The rotating flagellar filament primarily functions as a propeller, acting as an Archimedean screw, and supercoiling of the filament is essential as rotations of a straight filament do not generate thrust. Here, we show the atomic cryo-electron microscopy structures for flagellar filaments from enterohemorrhagic Escherichia coli O157:H7, enteropathogenic E. coli O127:H6, Achromobacter, and Sinorhizobium meliloti, where the outer domains dimerize or tetramerize to form either a sheath or a screw-like surface. A shared feature in all four structures is the formation of symmetrical homodimers between the outer domains of flagellin subunits, with one outer domain rotated 180° relative to the other. These symmetrical dimers are the result of outer domains being able to adopt either an “up” or “down” conformation.

The asymmetric unit (ASU) of the S. meliloti flagellar filament consists of two flagellin conformations, which are identical in the core domains, but the outer domains are rotated 180° from each other resulting in an “up” and a “down” conformation. The D2 domains in the S. meliloti filament form dimers between an arbitrary “up” conformation subunit (Sn) and two “down” conformation subunits (Sn + 5) and (Sn + 11) as depicted in Fig. 2b. Since the outer surface is bipolar, a “down” D2 will also interact with two “up” D2s. These interactions form a 3-start helix surrounding the flagellar core, which resembles the grooves in a helical screw. For the S. meliloti flagellar filament, a prominent 3-start helix is created by the outer domains surrounding the flagellar core, which gives the S. meliloti filament surface the appearance of a 3-start screw. The S. meliloti filament possesses a single outer domain, D2, while the ODS filaments have three outer domains, D2, D3 and D4. In positions with residue variations between FlaA and FlaB, there is support for FlaA at position 205 and FlaB at position 16 in both flagellins of the ASU. This suggests that there is likely a mixture of FlaA and FlaB in the flagellar filament segments of our images. A different behavior is observed for the unidirectional flagellar rotation in S. meliloti, which does not require a change in flagellar waveform during run-tumble transitions.

>MTSILTNNSAMAALSGVRSISSSMEDTQSRISSGLRVGSASDNAAYWSIATTMRSDNQALSAVQDALGLGAAKVDTAYSGMESAIEVVKEIKAKLVAATEDGVDKAKIQEEITQLKDQLTSIADAASFSGENWLQADLSGGAVTKSVVGSFVRDGSGSVAVKKVDYSLNANSVLFDTVGDTGILDKVYNVSQASVTLTVNTNGVESQHTVAAYSLESLTEAGAEFQGNYALQGGNSYVKVENVWVRAETAATGATGQEIAATTTAAGTITADSWVVDVGNAPAANVSAGQSVANINIVGMGAAALDALISGVDAALTDMTSAAASLGSISSRIDLQSEFVNKLSDSIESGVGRLVDADMNEESTRLKALQTQQQLAIQALSIANSDSQNVLSLFR[42x]> MANETEDHLESLICKVGEKSACSLESNLEGLAGVLEADLPNYKSKILRLLCTVARLLPEKLTIYTTLVGLLNARNYNFGGEFVEAMIRQLKESLKANNYNEAVYLVRFLSDLVNCHVIAAPSMVAMFENFVSVTQEEDVPQVRRDWYVYAFLSSLPWVGKELYEKKDAEMDRIFA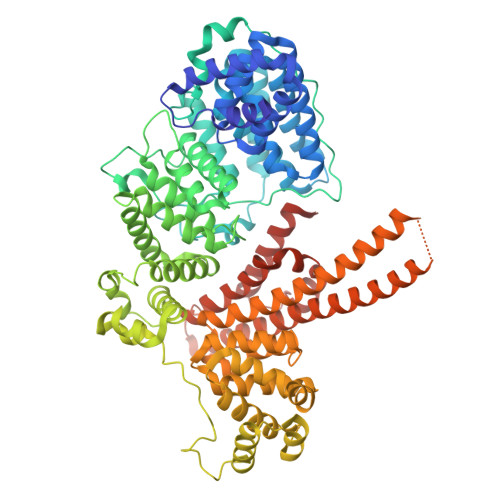NTESYLKRRQKTHVPMLQVWTADKPHPQEEYLDCLWAQIQKLKKDRWQERHILRPYLAFDSILCEALQHNLPPFTPPPHTEDSVYPMPRVIFRMFDYTDDPEGPVMPGSHSVERFVIEENLHCIIKSHWKERKTCAAQLVSYPGKNKIPLNYHIVEVIFAELFQLPAPPHIDVMYTTLLIELCKLQPGSLPQVLAQATEMLYMRLDTMNTTCVDRFINWFSHHLSNFQFRWSWEDWSDCLSQDPESPKPKFVREVLEKCMRLSYHQRILDIVPPTFSALCPVNPTCIYKYGDESSNSLPGHSVALCLAVAFKSKATNDEIFSILKDVPNPNQDDDDDEGFSFNPLKIEVFVQTLLHLAAKSFSHSFSALAKFHEVFKTLAESDEGKLHVLRVMFEVWRNHPQMIAVLVDKMIRTQIVDCAAVANWIFSSELSRDFTRLFVWEILHSTIRKMNKHVLKIQKELEEAKEKLARQHKRRSDDDDRSSDRKDGVLEEQIERLQEKVESAQSEQKNLFLVIFQRFIMILTEHLVRCETDGTSVLTPWYKNCIERLQQIFLQHHQIIQQYMVTLENLLFTAELDPHILAVFQQFCALQAAENLYFQGHHHHHH>[2x]GMIDEKFLIESNELVESSKIVMVGT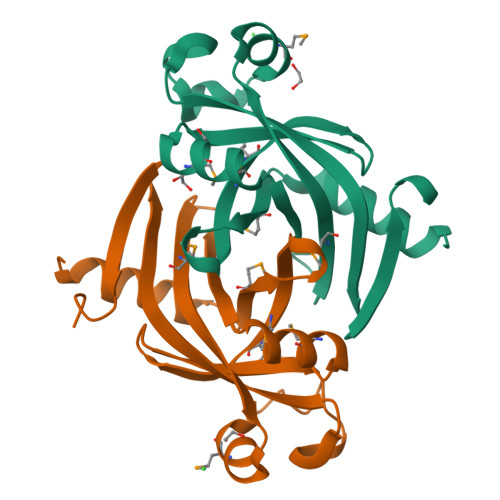NGENGYPNIKAMMRLKHDGLKKFWLSTNTSTRMVERLKKNNKICLYFVDDNKFAGLMLVGTIEILHDRASKEMLWTDGCEIYYPLGIDDPDYTALCFTAEWGNYYRHLKNITFKIDEIYNY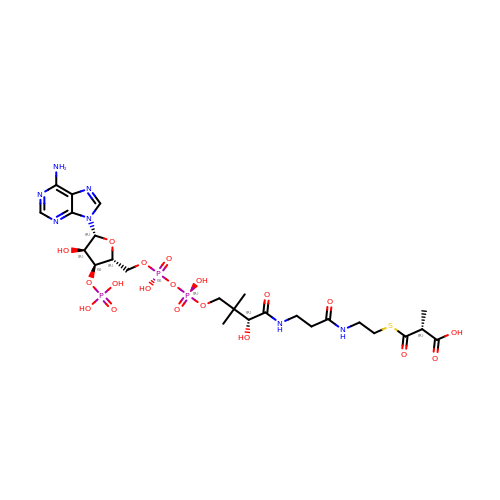METHYLMALONYL-COENZYME A | C25 H40 N7 O19 P3 S | MZFOKIKEPGUZEN-AGCMQPJKSA-N GcoA belongs to the CYP255A family of cytochrome P450 enzymes. Our recent characterization of a two-component P450 enzyme system consisting of a reductase, GcoB, and a P450 oxidase, GcoA, demonstrated that it demethylates diverse aromatic compounds, including guaiacol (which can be derived from coniferyl alcohol and represents the aromatic functionality of G-lignin that must undergo demethylation), guaethol, anisole (methoxybenzene), 2-methylanisole, and 3-methoxycatechol (3MC) with similar or greater efficiency than other O-aryl-demethylases described in the literature. However, GcoAB shows poor reactivity toward syringol, which can be derived from sinapyl alcohol via high-temperature reactions and represents the aromatic functionality of S-lignin that must undergo O-demethylation for further catabolism via ring-opening dioxygenases. In the present study, we hypothesized that substitution of GcoA-F169, which has the closest interaction with the bound substrate, may relax the specificity of the enzyme sufficiently to permit the O-demethylation of S-lignin type substrates.

The closest contact is with GcoA-F169, which forms a hydrophobic interaction with the C6 carbon on the aromatic ring of guaiacol. A broader survey of variants at the GcoA-F169 position (amino acids S, H, V, I, and L in addition to A) confirmed that GcoA-F169A exhibits the best catalytic performance in terms of both specific activity and reaction coupling, although other small side chains (S and V) also permitted reactivity with syringol, suggesting that these may permit syringol to assume a reactive conformation at the heme. Each protein variant also crystallized successfully with guaiacol and the structures showed that the orientation of the bound ligand remained consistent with that of the WT enzyme. Furthermore, comparison of the surrounding active site architecture confirmed no significant deviation from the WT.

> MTTTERPDLAWLDEVTMTQLERNPYEVYERLRAEAPLAFVPVLGSYVASTAEVCREVATSPDFEAVITPAGGRTFGHPAIIGVNGDIHADLRSMVEPALQPAEVDRWIDDLVRPIARRYLERFENDGHAELVAQYCEPVSVRSLGDLLGLQEVDSDKLREWFAKLNRSSTNAAVDENGEFANPEGFAEGDQAKAEIRAVVDPLIDKWIEHPDDSAISHWLHDGMPPGQTRDREYIYPTIYVYLLGAMQEPGHGMASTLVGLFSRPEQLEEVVDDPTLIPRAIAEGLRWTSPIWSATARISTKPVTIAGVDLPAGTPVMLSYGSANHDTGKYEAPSQYDLHRPPLPHLAFGAGNHACAGIYFANHVMRIALEELFEAIPNLERDTREGVEFWGWGFRGPTSLHVTWEV>[2x]MQNPQNLIWIDLEMTGLDPDRDVIIEMATIVTDSDLNTLAEGPVI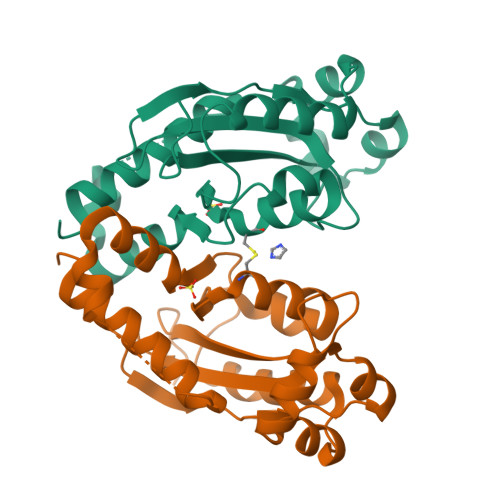AIHQPEEILAGMDEWNTRQHGQSGLTQRVRESTVSMAEAEAQTLAFLEQWVPKRSSPICGNSICQDRRFLYRHMPRLEGYFHYRNLDVSTLKELAARWAPQVRESFKKGNTHLALDDIRESIAELRHYRDHFIKL Dihydroxyacetone | C3 H6 O3 | 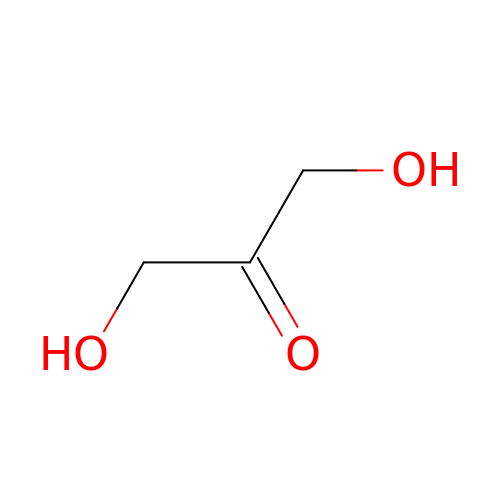RXKJFZQQPQGTFL-UHFFFAOYSA-N5-PHENYL-2-UREIDOTHIOPHENE-3-CARBOXAMIDE | C12 H11 N3 O2 S | 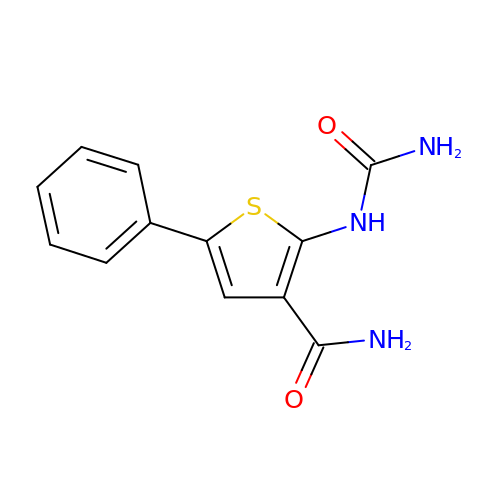PSVUSJKZJQMCSP-UHFFFAOYSA-N>PKTVRLNSLALFD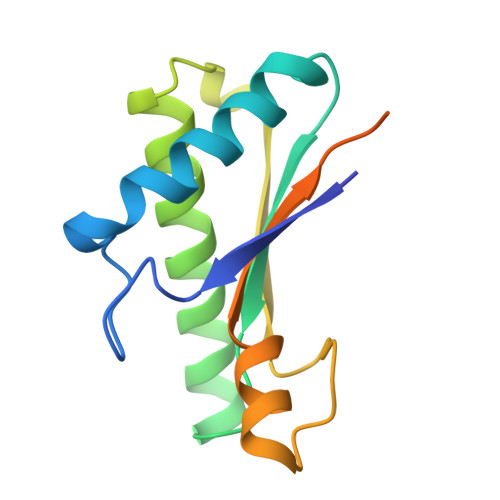AGKWTLKPGATKWLVNALVDIKAKAGWLIVVSGHTDNTGDPLRNQALSLKRAEAVRDWMRDTGDIPQSCFAVQGYGESRPVAPNDTAEGRARNRRVEISLVPQADACRLPDVSPAPEEGASENITE[3x]>MAAPVVAPPGVVVSRANKRSGAGPGGSGGGGARGAEEEPPPPLQAVLVADSFDRRFFPISKDQPRVLLPLANVALIDYTLEFLTATGVQETFVFCCWKAAQIKEHLLKSKWCRPTSLNVVRIITSELYRSLGDVLRDVDAKALVRSDFLLVYGDVISNINITRALEEHRLRRKLEKNVSVMTMIFKESSPSHPTRCHEDNVVVAVDSTTNRVLHFQKTQGLRRFAFPLSLFQGSSDGVEVRYDLLDCHISICSPQVAQLFTDNFDYQTRDDFVRGLLVNEEILGNQIHMHVTAKEYGARVSNLHMYSAVCADVIRRWVYPLTPEANFTDSTTQSCTHSRHNIYRGPEVSLGHGSILEENVLLGSGTVIGSNCFITNSVIGPGCHIGDNVVLDQTYLWQGVRVAAGAQIHQSLLCDNAEVKERVTLKPRSVLTSQVVVGPNITLPEGSVISLHPPDAEEDEDDGEFSDDSGADQEKDKVKMKGYNPAEVGAAGKGYLWKAAGMNMEEEEELQQNLWGLKINMEEESESESEQSMDSEEPDSRGGSPQMDDIKVFQNEVLGTLQRGKEENISCDNLVLEINSLKYAYNISLKEVMQVLSHVVLEFPLQQMDSPLDSSRYCALLLPLLKAWSPVFRNYIKRAADHLEALAAIEDFFLEHEALGISMAKVLMAFYQLEILAEETILSWFSQRDTTDKGQQLRKNQQLQRFIQWLKEAEEESSEDD[2x];>MHHHHHHGGGSENLYFQSPGSAAKGSELSERIESFVETLKRGGGPRSSEEMARETLGLLRQIITDHRWSNAGELMELIRREGRRMTAAQPSETTVGNMVRRVLKIIREEYGRLHGRSDESDQQESLHKLLTSGGLNEDFSFHYAQLQSNIIEAINELLVELEGTMENIAAQALEHIHSNEVIMTIGFSRTVEAFLKEAARKRKFHVIVAECAPFCQGHEMAVNLSKAGIETTVMTDAAIFAVMSRVNKVIIGTKTILANGALRAVTGTHTLALAAKHHSTPLIVCAPMFKLSPQFPNEEDSFHKFVAPEEVLPFTEGDILEKVSVHCPVFDYVPPELITLFISNIGGNAPSYIYRLMSELYHPDDHVL[2x];>[2x]MAAVAVAVREDSGSGMKAELPPGPGAVGREMTKEEKLQLRKEKKQQKKKRKEEKGAEPETGSAVSAAQCQVGPTRELPESGIQLGTPREKVPAGRSKAELRAERRAKQEAERALKQARKGEQGGPPPKASPSTAGETPSGVKRLPEYPQVDDLLLRRLVKKPERQQVPTRKDYGSKVSLFSHLPQYSRQNSLTQFMSIPSSVIHPAMVRLGLQYSQGLVSGSNARCIALLRALQQVIQDYTTPPNEELSRDLVNKLKPYMSFLTQCRPLSASMHNAIKFLNKEITSVGSSKREEEAKSELRAAIDRYVQEKIVLAAQAISRFAYQKISNGDVILVYGCSSLVSRILQEAWTEGRRFRVVVVDSRPWLEGRHTLRSLVHAGVPASYLLIPAASYVLPEVSKVLLGAHALLANGSVMSRVGTAQLALVARAHNVPVLVCCETYKFCERVQTDAFVSNELDDPDDLQCKRGEHVALANWQNHASLRLLNLVYDVTPPELVDLVITELGMIPCSSVPVVLRVKSSDQ;>[2x]MDDKELIEYFKSQMKEDPDMASAVAAIRTLLEFLKRDKGETIQGLRANLTSAIETLCGVDSSVAVSSGGELFLRFISLASLEYSDYSKCKKIMIERGELFLRRISLSRNKIADLCHTFIKDGATILTHAYSRVVLRVLEAAVAAKKRFSVYVTESQPDLSGKKMAKALCHLNVPVTVVLDAAVGYIMEKADLVIVGAEGVVENGGIINKIGTNQMAVCAKAQNKPFYVVAESFKFVRLFPLNQQDVPDKFKYKADTLKVAQTGQDLKEEHPWVDYTAPSLITLLFTDLGVLTPSAVSDELIKLYL;>MEFQAVVMAVGGGSRMTDLTSSIPKPLLPVGNKPLIWYPLNLLERVGFEEVIVVTTRDVQKALCAEFKMKMKPDIVCIPDDADMGTADSLRYIYPKLKTDVLVLSCDLITDVALHEVVDLFRAYDASLAMLMRKGQDSIEPVPGQKGKKKAVEQRDFIGVDSTGKRLLFMANEADLDEELVIKGSILQKHPRIRFHTGLVDAHLYCLKKYIVDFLMENGSITSIRSELIPYLVRKQFSSASSQQGQEEKEEDLKKKELKSLDIYSFIKEANTLNLAPYDACWNACRGDRWEDLSRSQVRCYVHIMKEGLCSRVSTLGLYMEANRQVPKLLSALCPEEPPVHSSAQIVSKHLVGVDSLIGPETQIGEKSSIKRSVIGSSCLIKDRVTITNCLLMNSVTVEEGSNIQGSVICNNAVIEKGADIKDCLIGSGQRIEAKAKRVNEVIVGNDQLMEI[2x];> PGLSCRFYQHKFPEVEDVVMVNVRSIAEMGAYVSLLEYNNIEGMILLSELSRRRIRSINKLIRIGRNECVVVIRVDKEKGYIDLSKRRVSPEEAIKCEDKFTKSKTVYSILRHVAEVLEYTKDEQLESLFQRTAWVFDDKYKRPGYGAYDAFKHAVSDPSILDSLDLNEDEREVLINNINRRLTPQAVKIRADIEVACYGYEGIDAVKEALRAGLNCSTENMPIKINLIAPPRYVMTTTTLERTEGLSVLSQAMAVIKEKIEEKRGVFNVQMEPKVVTDTDETELARQMERLERENAEVDGDDDAEEMEAKAED;> MAGGEAGVTLGQPHLSRQDLTTLDVTKLTPLSHEVISRQATINIGTIGHVAHGKSTVVKAISGVHTVRFKNELERNITIKLGYANAKIYKLDDPSCPRPECYRSCGSSTPDEFPTDIPGTKGNFKLVRHVSFVDCPGHDILMATMLNGAAVMDAALLLIAGNESCPQPQTSEHLAAIEIMKLKHILILQNKIDLVKESQAKEQYEQILAFVQGTVAEGAPIIPISAQLKYNIEVV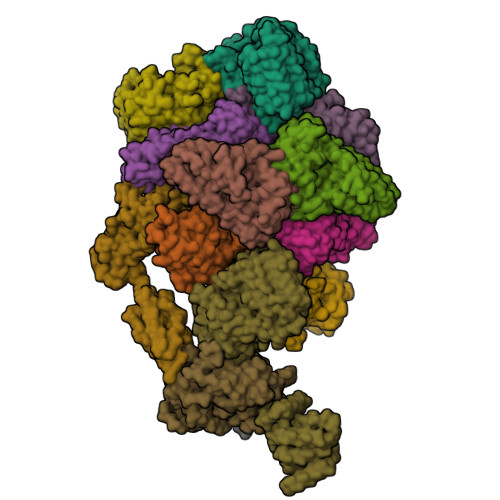CEYIVKKIPVPPRDFTSEPRLIVIRSFDVNKPGCEVDDLKGGVAGGSILKGVLKVGQEIEVRPGIVSKDSEGKLMCKPIFSKIVSLFAEHNDLQYAAPGGLIGVGTKIDPTLCRADRMVGQVLGAVGALPEIFTELEISYFLLRRLLGVRTEGDKKAAKVQKLSKNEVLMVNIGSLSTGGRVSAVKADLGKIVLTNPVCTEVGEKIALSRRVEKHWRLIGWGQIRRGVTIKPTVDDD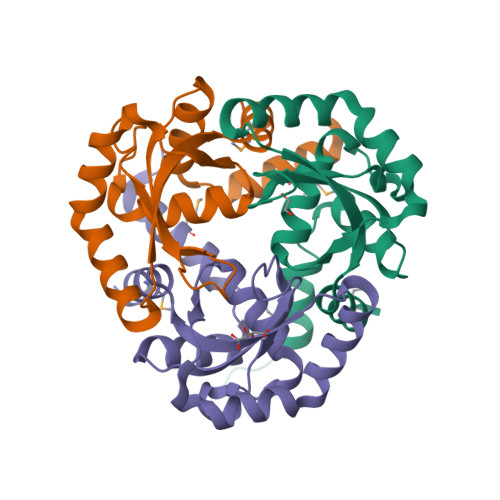>[3x]GSMLHGLKQRLEALHHPGELEGSPQNLHQLLGVSIEQSVPQAQTMLVERHLASLTGDEARLLAALSDGSAFALLTLYSGSRFSRGEVLYRYSNAGRAAGIQCNDFIALYLNHLFAQGLVIASDFTESLRTDYELCEGDSDFRKAQAELQIHLPKLSIRRETLRISPLGRQLWTLMTTPADIEEGH> GAMEGIKVFLHERELWLKFHEVGTEMIITKAGRRMFPSYKVKVTGLN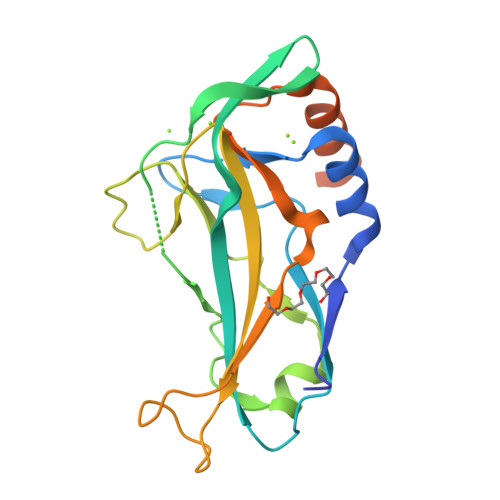PKTKYILLMDIVPADDHRYKFADNKWSVTGKAEPAMPGRLYVHPDSPATGAHWMRQLVSFQKLKLTNNHLDPFGHIILNSMHKYQPRLHIVKADENNGFGSKNTAFCTHVFPETAFIAVTSYQNHKITQLKIENNPFAKGFRGSDDMELHRMSRMQ~{tert}-butyl (2'~{S},3~{S})-2-oxidanylidene-2'-phenyl-spiro[1~{H}-indole-3,3'-pyrrolidine]-1'-carboxylate 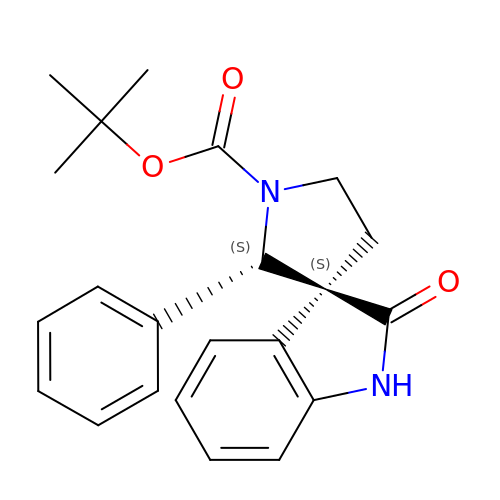| C22 H24 N2 O3 | FXVLEOBGAHQNAI-AVRDEDQJSA-N> KFIYGDVDGNGSVRSIDAVLIRDYV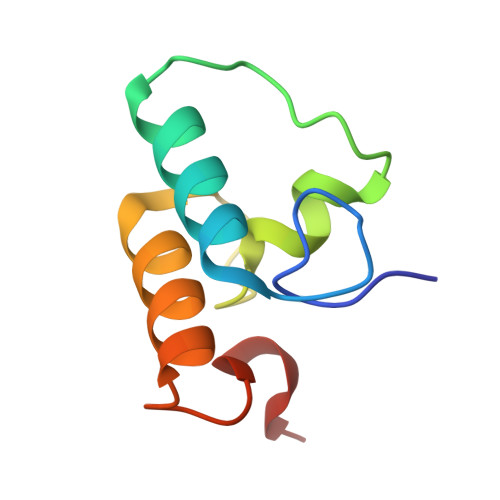LGKINEFPYEYGMLAADVDGNGSIKINDAVLVRDYVLGKIFLFPVEEKEE> SNISRQAYADMFGPTVGDKVRLADTELWIEVEDDLTTYGEEVKFGGGKVIRDGMGQGQMLAADCVDLVLTNALIVDHWGIVKADIGVKDGRIFAIGKAGNPDIQPNVTIPIGAATEVIAAEGKIVTAGGIDTHIHWICPQQAEEALVSGVTTMVGGGTGPAAGTHATTCTPGPWYISRMLQAADSLPVNIGLLGKGNVSQ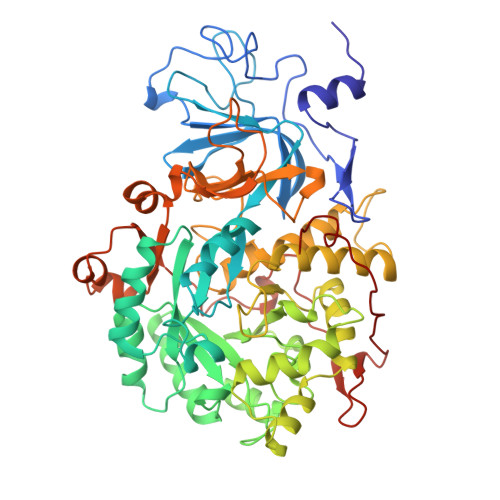PDALREQVAAGVIGLAIHEDWGATPAAIDCALTVADEMDIQVALHSDTLNESGFVEDTLAAIGGRTIHTFHTEGAGGGHAPDIITACAHPNILPSSTNPTLPYTLNTIDEHLDMLMVCHHLDPDIAEDVAFAESRIRRETIAAEDVLHDLGAFSLTSSDSQAMGRVGEVILRTWQVAHRMKVQRGALAEETGDNDNFRVKRYIAKYTINPALTHGIAHEVGSIEVGKLADLVVWSPAFFGVKPATVIKGGMIAIAPMGDINASIPTPQPVHYRPMFGALGSARHHCRLTFLSQAAAANGVAERLNLRSAIAVVKGCRTVQKADMVHNSLQPNITVDAQTYEVRVDGELITSEPADVLPMAQRYFLF>[2x]QMNYEEVIKKYK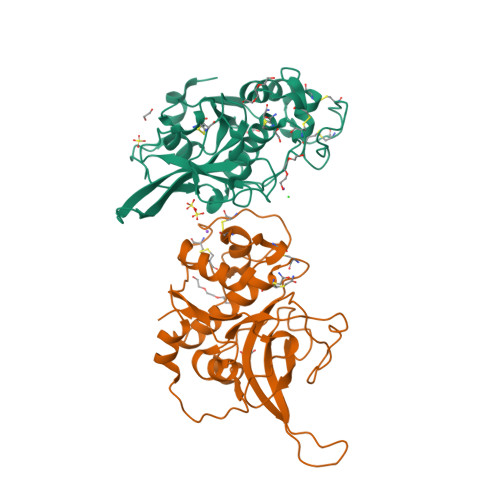GNENFDHAAYDWRLHSGVTPVKDQKNCGSCWAFSSIGSVESQYAIRKNKLITLSEQELVDCSFKNYGCNGGLINNAFEDMIELGGICTDDDYPYVSDAPNLCNIDRCTEKYGIKNYLSVPDNKLKEALRFLGPISISVAVSDDFAFYKEGIFDGECGDQLNHAVMLVGFGMKEIVNPLTKKGEKHYYYIIKNSWGQQWGERGFINIETDESGLMRKCGLGTDAFIPLIE>MSNDDNVELTDGFHVLIDALKMNDIDTMYGVVGIPITNLARMWQDDGQRFYSFRHEQHAGYAASIAGYIEGKPGVCLTVSAPGFLNGVTSLAHATTNCFPMILLSGSSEREIVDLQQGDYEEMDQMNVARPHCKASFRINSIKDIPIGIARAVRTAVSGRPGGV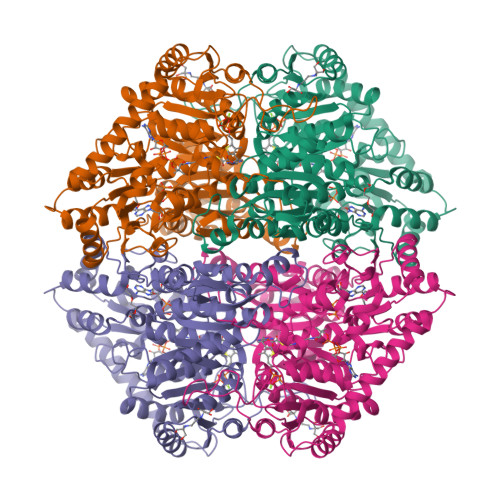YVDLPAKLFGQTISVEEANKLLFKPIDPAPAQIPAEDAIARAADLIKNAKRPVIMLGKGAAYAQCDDEIRALVEETGIPFLPMGMAKGLLPDNHPQSAAATRAFALAQCDVCVLIGARLNWLMQHGKGKTWGDELKKYVQIDIQANEMDSNQPIAAPVVGDIKSAVSLLRKALKGAPKADAEWTGALKAKVDGNKAKLAGKMTAETPSGMMNYSNSLGVVRDFMLANPDISLVNEGANALDNTRMIVDMLKPRKRLDSGTWGVMGIGMGYCVAAAAVTGKPVIAVEGDSAFGFSGMELETICRYNLPVTVIIMNNGGIYKGNEADPQPGVISCTRLTRGRYDMMMEAFGGKGYVANTPAELKAALEEAVASGKPCLINAMIDPDAGVESGRIKSLNVVSKVGKK[2x]>MNAHHHHHHGSAENLYFQGHHVSITGMQDCVQLDQYTLKDEIGKGSYGVVKLAYNENDNTYYAMKVLSKKKLIRQAGGCIQPRGPIEQVYQEIAIL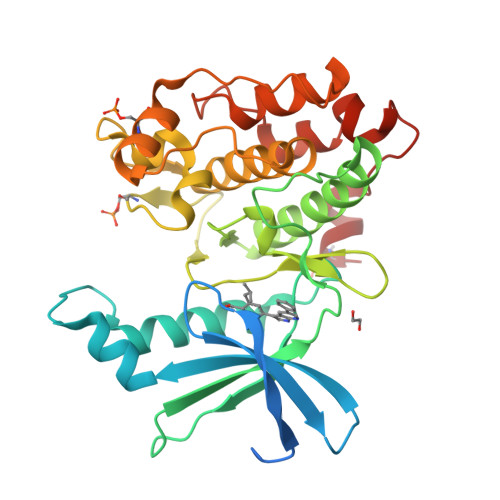KKLDHPNVVKLVEVLDDPNEDHLYMVFELVNQGPVMEVPTLKPLSEDQARFYFQDLIKGIEYLHYQKIIHRDIKPSNLLVGEDGHIKIADFGVSNEFKGSDALLSNTVGTPAFMAPESLSETRKIFSGKALDVWAMGVTLYCFVFGQCPFMDERIMCLHSKIKSQALEFPDQPDIAEDLKDLITRMLDKNPESRIVVPEIKLHPWVTRHGAEPLPSEDENCTLVE[2x]>MGLMSKEQLIILAKNSSPKEGEYKKILELLDEYNLLNNSVEKNSIDLYLKLNELSKSIDIYLKKYKNSKRNNALYQLKSDLTKEVIEIKDTNLKPLEKNIHFVWVGGMINNISIDYINQWKDINSDYETIIWYDSEALLVNILKKAIIDSSNKEVLTKYESVLNDNSFDSNKFYRERMEVIFRKQKEFNNYYNTNDNYTKSLNDVIKVYLIEKYLKTDEELEKYINESKEVFKANGAKDIREYDILDDVELKSIYEQELLMRFNLAS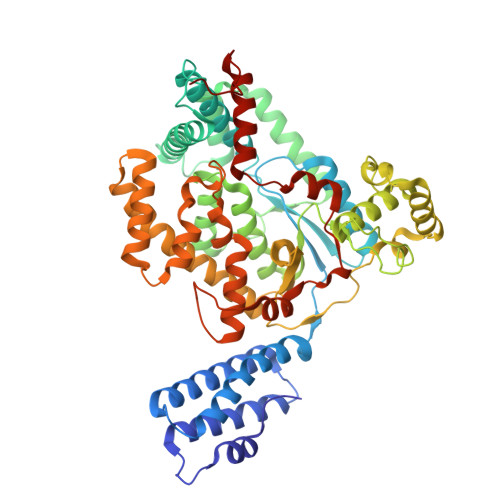ASDIIRVIVLNKLGGIYLDVDVLPGIKKHIFKDINKPTNISENKWQMIQLETIMKYKQYIKGYTENSFKNLPSDLQEMLQEKVVEKNLKSDIFQRLGDIFISELDTKIAFMFGKIANQVLISKKNSYSLNLIINQIKNRYNIINKCLSSAIEKGSNFNNTVDIFIQQLNEFYVNEGFFVSKVMGYLGDGYMPDMRATLNISGPGIYTAAYYDLLYFNERSLNPQILQEDLKYFEVPQALISQQTEQEINSSWTFNQVKSQIEYKKLVEKYTNKSLSLEHHHHHH[2x]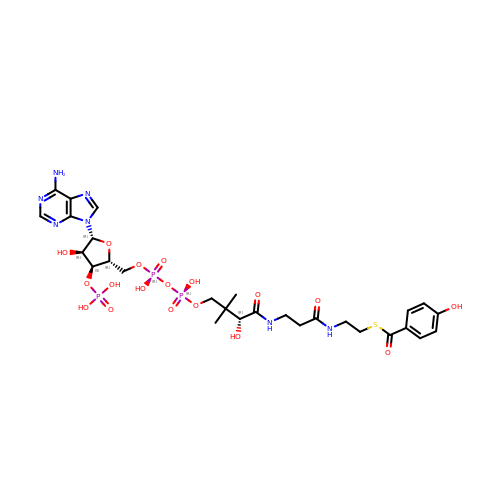4-HYDROXYBENZOYL COENZYME A | C28 H40 N7 O18 P3 S | LTVXPVBFJBTNIJ-TYHXJLICSA-N>GPKKISNCSKIHLSTKLLAVDFPAHFVKSISCQICEHILADPVETSCKHLFCRICILRCLKVMGSYCPSCRYPCFPTDLESPVKSFLNILNSLMVKCPAQDCNEEVSLEKYNHHVSSHKESKETLVHINKGGRPRQHLLSLTRRAQKHRLRELKIQVKEFADKEEGGDVKAVCLTLFLLALRARNEHRQADELEAIMQGRGSGLQPAVCLAIRVNTFLSCSQYHKMYRTVKAITGRQIFQPLHALRNAEKVLLPGYHPFEWQPPLKNVSSRTDVGIIDGLSGLASSVDEYPVDTIAKRFRYDSALVSALMDMEEDILEGMRSQDLDDYLNGPFTVVVKESCDGMGDVSEKHGSGPAVPEKAVRFSFTVMRITIEHGSQNVKVFEEPKPNSVLCCKPLCLMLADESDHETLTAILSPLIAEREAMKSSELTLEMGGIPRTFKFIFRGTGYDEKLVREVEGLEASGSVYICTLCDTTRLEASQNLVFHSITRSHAENLQRYEVWRSNPYHESVEELRDRVKGVSAKPFIETVP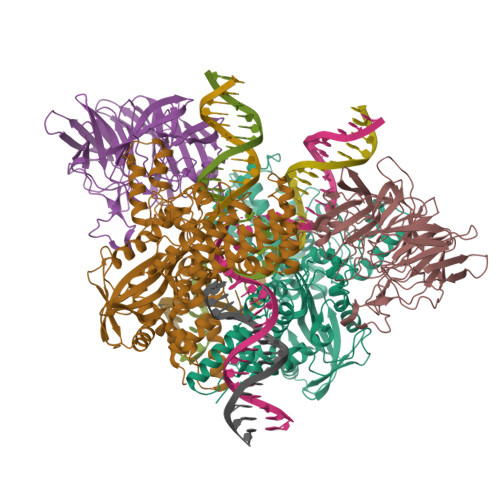SIDALHCDIGNAAEFYKIFQLEIGEVYKHPNASKEERKRWQATLDKHLRKRMNLKPIMMMNGNFARKLMTQETVDAVCELIPSEERHEALRELMDLYLKMKPVWRSSCPAKECPESLCQYSFNSQRFAELLSTKFKYRYEGKITNYFHKTLAHVPEIIERDGSIGAWASEGNESGNKLFRRFRKMNARQSKCYEMEDVLKHHWLYTSKYLQKFMNAHNA[2x];>[2x]GPMALQMVTVGHNIALIQPGFSLMNFDGQVFFFGQKGWPKRSCPTGVFHFDIKQNHLKLKPAIFSKDSCYLPPLRYPATCSYKGSIDSDKHQYIIHGGKTPNNELSDKIYIMSVACKNNKKVTFRCTEKDLVGDVPEPRYGHSIDVVYSRGKSMGVLFGGRSYMPSTQRTTEKWNSVADCLPHVFLIDFEFGCATSYILPELQDGLSFHVSIARNDTVYILGGHSLASNIRPANLYRIRVDLPLGTPAVNCTVLPGGISVSSAILTQTNNDEFVIVGGYQLENQKRMVCSLVSLGDNTIEISEMETPDWTSDIKHSKIWFGSNMGNGTIFLGIPGDNKQAMSEAFYFYTLRCSEEDLSEDQKI~{N}1-[(~{Z},3~{R})-4-[2-(3-methoxyphenyl)propan-2-ylamino]-3-oxidanyl-1-phenyl-but-1-en-2-yl]-5-piperidin-1-yl-~{N}3,~{N}3-dipropyl-benzene-1,3-dicarboxamide | C39 H52 N4 O4 | 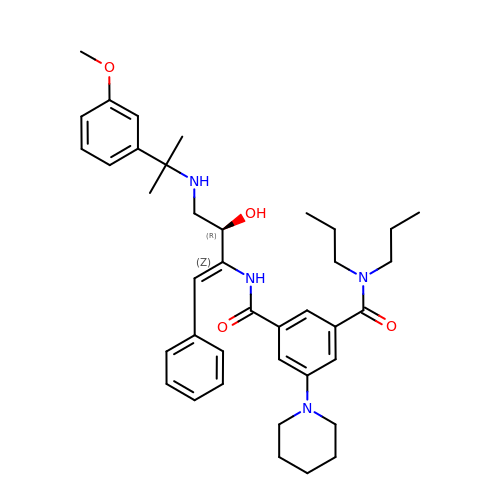UCBMZABMPAPJRC-LMOGZCTNSA-N> MTVTRRHFLKLSAGAAVAGAFTGLGLSLAPTVARAELQKLQWAKQTTSICCYCAVGCGLIVHTAKDGQGRAVNVEGDPDHPINEGSLCPKGASIFQLGENDQRGTQPLYRAPFSDTWKPVTWDFALTEIAKRIKKTRDASFTEKNAAGDLVNR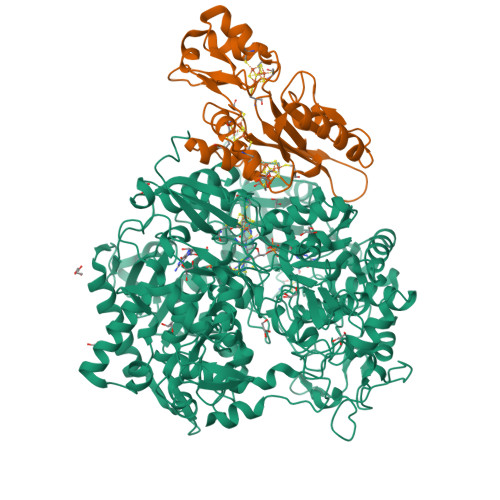TEAIASFGSAAMDNEECWAYGNILRSLGLVYIEHQARIUHSPTVPALAESFGRGAMTNHWNDLANSDCILIMGSNAAENHPIAFKWVLRAKDKGATLIHVDPRFTRTSARCDVYAPIRSGADIPFLGGLIKYILDNKLYFTDYVREYTNASLIVGEKFSFKDGLFSGYDAANKKYDKSMWAFELDANGVPKRDPALKHPRCVINLLKKHYERYNLDKVAAITGTSKEQLQQVYKAYAATGKPDKAGTIMYAMGWTQHSVGVQNIRAMAMIQLLLGNIGVAGGGVNALRGESNVQGSTDQGLLAHIWPGYNPVPNSKAATLELYNAATPQSKDPMSVNWWQNRPKYVASYLKALYPDEEPAAAYDYLPRIDAGRKLTDYFWLNIFEKMDKGEFKGLFAWGMNPACGGANANKNRKAMGKLEWLVNVNLFENETSSFWKGPGMNPAEIGTEVFFLPCCVSIEKEGSVANSGRWMQWRYRGPKPYAETKPDGDIMLDMFKKVRELYAKEGGAYPAPIAKLNIADWEEHNEFSPTKVAKLMNGYFLKDTEVGGKQFKKGQQVPSFAFLTADGSTCSGNWLHAGSFTDAGNLMARRDKTQTPEQARIGLFPNWSFCWPVNRRILYNRASVDKTGKPWNPAKAVIEWKDGKWVGDVVDGGGDPGTKHPFIMQTHGFGALYGPGREEGPFPEHYEPLECPVSKNPFSKQLHNPVAFQIEGEKKAVCDPRYPFIGTTYRVTEHWQTGLMTRRCAWLVEAEPQIFCEISKELAKLRGIGNGDTVKVSSLRGALEAVAIVTERIRPFKIEGVDVHMVGLPWHYGWMVPKNGGDTANLLTPSAGDPNTGIPETKAFMVDVRKVWSHP;> MGKMFFVDLSRCTACRGCQIACKQWKNLPAEETRNTGSHQNPPDLSYVTLKTVRFTEKSRKGPGIDWLFFPEQCRHCVEPPCKGQADVDLEGAVVKDETTGAVLFTELTAKVDGESVRSACPYDIPRIDPVTKRLSKCDMCNDRVQNGLLPACVKTCPTGTMNFGDEQEMLALAEKRLAEVKKTYPGAVLGDPNDVRVVYLFTRDPKDFYEHAVADLAPSMMTRQQLFARLFRPRA>GIGTGFPFDPHYVEVLGERMHYVDVGPRDGTPVLFLHGNPTSSYVWRNIIPHVAPTHRCIAPDLIGMGKSDKPDLGYFFDDHVRFMDAFIEALGLEEVVLVIHDWGSALGFHWAKRNPERVKGIAFMEFIRPIPTWDEWPEFARETFQAFRTTDVGRKLIIDQNVFIEGTLPMGVVRPLTEVEMDHYREPFLNPVDREPLWRFPNELPIAGEPANIVALVEEYMDWLHQSPVPKLLFWGTPGVLIPPAEAARLAKSLPNCKAVDIGPGLNLLQEDNPDLIGSEIARWLSTLEI[2x]

The specific and covalent labeling of the protein HaloTag with fluorescent probes in living cells makes it a powerful tool for bioimaging. However, the irreversible attachment of the probe to HaloTag precludes imaging applications that require transient binding of the probe and comes with the risk of irreversible photobleaching. Here, we introduce exchangeable ligands for fluorescence labeling of HaloTag (xHTLs) that reversibly bind to HaloTag and that can be coupled to rhodamines of different colors. Here, we introduce exchangeable HaloTag Ligands (xHTLs) for the reversible fluorescence labeling of HaloTag7 with rhodamines, opening up new possibilities in bioimaging for a powerful labeling tool.

Taking advantage of the crystal structure of HaloTag7 labeled with tetramethylrhodamine (TMR), we used computational screening to identify tentative xHTLs. In brief, putative xHTLs were designed by varying the terminal alkane chain length (C4–C7) as well as by replacing the chlorine atom with other functional groups. TMR-linked PEG2-C5-methylsulfonamide (S5) was one of the compounds that presented a lower ΔGbind compared to regular TMR-CA (ΔΔGbind = −4.2 kcal/mol), which displays a KD < 1 μM.6 We synthesized S5 as well as a fluorinated triflamide derivative T5 in order to improve cell permeability and coupled both to fluorogenic rhodamine dyes−34 such as SiR35. The binding mode of TMR-S5 and TMR-T5 to HaloTag7 was further studied through X-ray crystallography. While the S5 moiety occupies a similar position in both the docking experiment and the crystal structure (rmsd = 1.0 ± 0.3 Å on five atoms), the TMR shows a different position on the HaloTag7 surface in the docking experiment. The alkane-PEG chain occupies the same hydrophobic channel but presents a different conformation. The L209/I211 conformational change induced by the TMR-T5 binding in the HaloTag7 active site allows a more favorable orientation of the sulfonamide group to form hydrogen bonds with active side residues than observed for TMR-S5; while the TMR-S5 nitrogen-sulfonamide forms a 3.3 Å hydrogen bond with the catalytic D106 carboxylic acid moiety, the corresponding hydrogen bond in bound TMR-T5 is only 2.7 Å. This difference in binding interactions might contribute to the higher affinity of T5-based probes than those of S5-based probes. In contrast, SiR- S5 showed only a 2-fold fluorescence increase upon HaloTag7 binding.>MVLDGPYQPVAFKP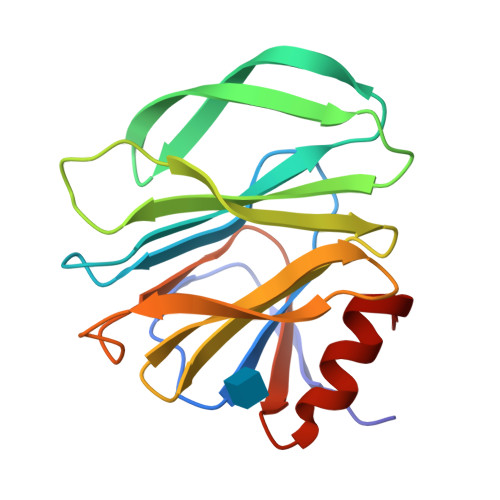PNDYWILVNSNSNGVVLEGTNNTDVWVAIISIEPNVNSESRQYSLFGVNKQITVVNTSNKWKFMEMFRNNSNAEFQHKRTLTSSTKLVGILKHGGRLWTYHGETPNATTDYSTTSNLNEISVTTYAEFYIIPRSQESKCTEYINTGL[8x]> TVGCVAVDSHGNLASATSTGGLVNKMVGRIGDTPLIGAGTYANELCAVSATGKGE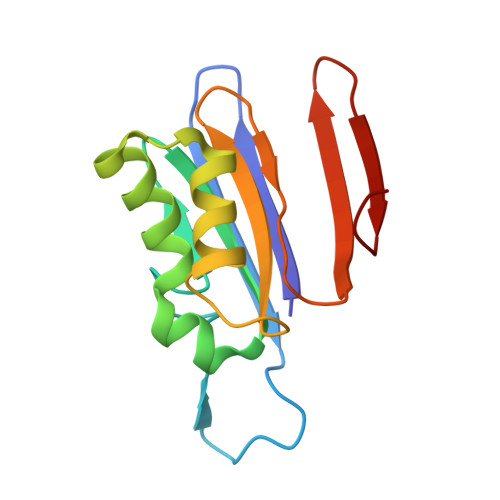EIIRATVARDVAALMEFKGLSLKEAADFVIHERTPKGTVGLIAVSAAGEIAMPFNTTGMFRACATEDGYSEIAIWPTT> MPSPTTVPVATAGRLAEPYIDPAAQVHAIASIIGDVRIAAGVRVAAGVSIRADEGAPFQVGKESILQEGAVIHGLEYGRVLGDDQADYSVWIGQRVAITHKALIHGPAYLGDDCFVGFRSTVFNARVGAGSVIMMHALVQDVEIPPGRYVPSGAIITTQQQADRLPEVRPEDREFARHIIG

β-Carboxysome biogenesis is reliant on the protein CcmM as a central organizing scaffold. The full-length CcmM protein in Synechococcus elongatus PCC 7942 (Se7942) is a homotrimer of ~58-kDa subunits (SeM58). The N terminus of each M58 protomer consists of a γ-class carbonic anhydrase-like (γCAL) domain that has lost the functional motifs for CA activity, followed by three Rubisco small subunit-like (SSUL) modules connected by flexible linkers. The γCAL domains mediate M58 trimer formation.

The asymmetric unit of the crystal contained the protomer of γCAL181, while γCAL exists as a trimer in solution. Indeed, analysis using proteins, interfaces, structures and assemblies (PISA)48 indicated an extensive interface between subunits (4,180 Å2 buried at the interface from a total accessible surface of 18,860 Å2). Thus, a total of six salt bridges stabilizes the dimer of γCAL trimers. Note that γCAL198 and γCAL181 are nevertheless trimeric in solution, suggesting that the head-to-head association occurs only at high protein concentrations within the condensate or crystal. To investigate the functional relevance of this interaction, we disrupted the salt bridges by either mutating R164 to aspartate or D172 to lysine. Strikingly, both R164D and D172K mutants strongly reduced homodemixing of M58, indicating that dimer-of-trimer formation via the γCAL domains provides critical valency, presumably by increasing the local concentration of SSUL modules.>[2x]GVHLPDDETFTSYYPAAGNDELIGALKSAASGDGVQAIYLWGPVKSGRTHLIHAACARANELERRSFYIPLGIHASISTALLEGLEQFDLIC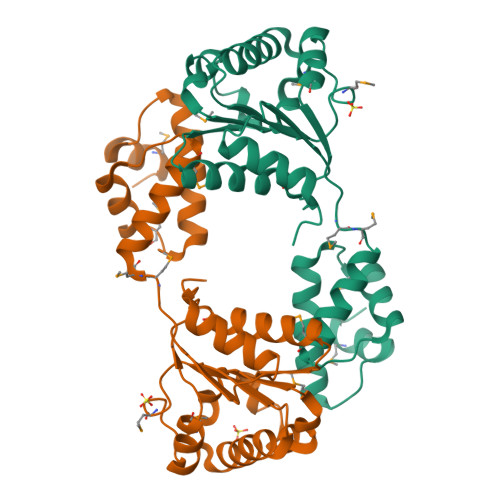IDDVDAVAGHPLWEEAIFDLYNRVAEQKRGSLIVSASASPMEAGFVLPDLVSRMHWGLTYQLQPMMDDEKLAALQRRAAMRGLQLPEDVGRFLLNRMARDLRTLFDVLDRLDKASMVHQRKLTIPFVKEMLRL> SHMGQGGSNPKFENIAEGLRALLARSHVERTTDEGTWVAGVFVYGGSKTSLYNLRRGTALAIPQCRLTPLSRLPFGMAPGPGPQPGPLRESIVCYFMVFLQTHIFAEVLK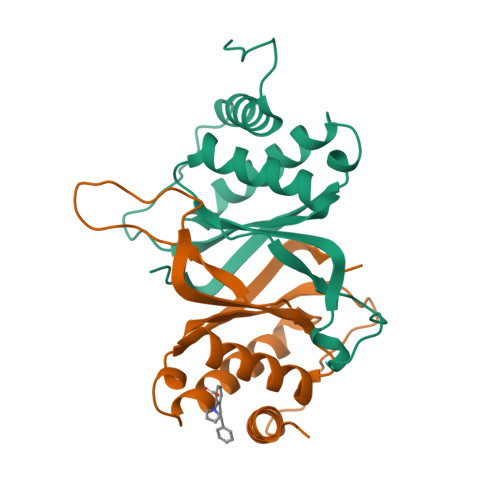DAIKDLVMTKPAPTCNIRVTVCSFDDGVDLP;> SNPKFENIAEGLRALLARSHVERTTDEGTWVAGVFVYGGSKTSLYNLRRGTALAIPQCRLTPLSRLPFGMAPGPGPQPGPLRESIVCYFMVFLQTHIFAEVLKDAIKDLVMTKPAPTCNIRVTVCSFDDGVDLP> 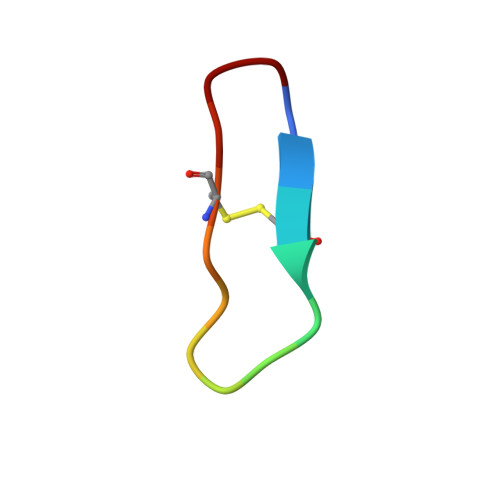GRCTKSRPPICFPD L-alanyl-N-[(1S,2R)-1-benzyl-2-hydroxypropyl]-L-alaninamide 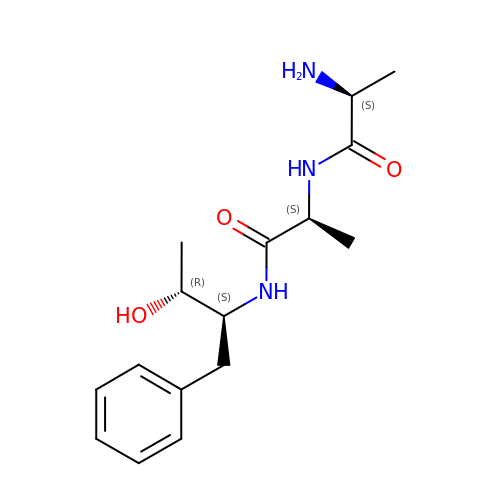| C16 H25 N3 O3 | CPAOOGAUUDSJCS-FMSGJZPZSA-N TP901-1 is a temperate bacteriophage of Lactococcus lactis that enters either the lytic or the lysogenic lifecycle when infecting a bacterium. In the TP901-1 bacteriophage a genetic switch exist, and is regulated by two divergently oriented promoters PL and PR, three operator sites on the DNA (OD, distant located operator; OL, left operator; OR, right operator) and two proteins, the Modulator of Repression (MOR) and the repressor, CI (known as Clear I in λ phage). CI from TP901-1 consists of an NTD responsible for DNA binding and a CTD responsible for oligomerization. The full-length protein has been shown to be a hexamer in solution, where CTD is responsible for the oligomerization state of the protein.

Co-crystallization experiments with DNA were also carried out both with CI∆58 and CI∆43. One of the crystals diffracted significantly better, however turned out to contain only protein (DNA was absent). Furthermore residues beyond Val80 were not visible suggesting that the better diffracting crystals were obtained because of limited proteolysis occurring during the long crystallization period. The resulting crystal structure is essentially the CI-NTD domain, well described in12, but contains six additional C-terminal residues compared to the previous structure, and is hereon denoted NTD80. The six additional residues mainly consist of hydrophobic amino acids and interact closely with the rest of the domain. The extended region is stabilized by hydrogen bonds of the Phe75 backbone carbonyl oxygen with the side chain of Arg8 and the backbone amide of Val77 as well as Met79 π-interactions with Trp71 and a hydrogen bond between the carbonyl group of Met79 and the backbone N of Ser68 (see Table S2 for statistics). The extended CI-NTD crystal structure as well as the NMR relaxation data also precisely identifies residues 81–89 of TP901-1 CI as a flexible linker, while residues 75–80 should be included in the CI-NTD. The crystal structure of the CI-NTD fits well within the envelope in terms of dimensions. Next, we generated a large pool of possible conformers (400.000 copies) using the crystal structure of CI-NTD80 and the model of the dimerization region. The MOR binding has been suggested to take place in a region including part of the scaffolding helix (α2), and a region including the last two helices of NTD.

> MQTDTSNRLKQIMAERNLKQVDILNLSIPFQKKFGIKLSKSTLSQYVNSVQSPDQNRIYLLAKTLGVSEAWLMGFDVPMV>[2x]MGSSTGFHHADHVNYSSNLNKEEILEQLLLSYEGLSDGQVNWVC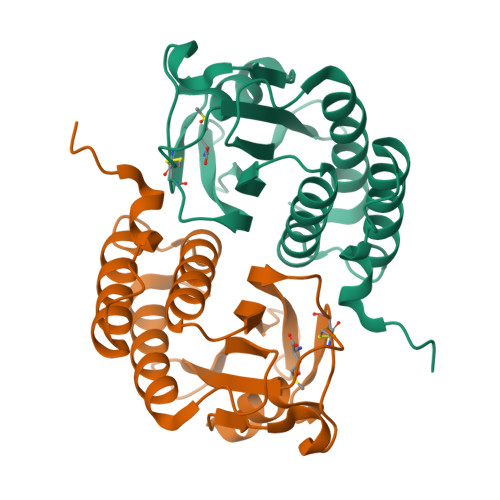NLSNASSLIWHAYKSLAVDINWAGFYVTQASEENTLILGPFQGKVACQMIQFGKGVCGTAASTKETQIVPDVNKYPGHIACDGETKSEIVVPIISNDGKTLGVIDIDCLDYEGFDHVDKEFLEKLAKLINKSCVFK> VD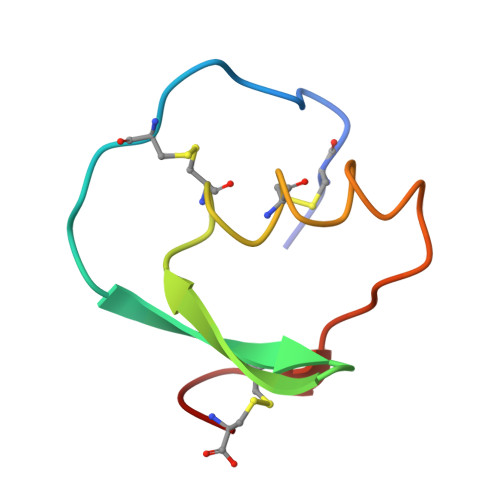CSEYPKPACTDEYRPLCGSDNKTYGNKCNFCNAVVESNGTLTLSHFGKC>AKPDRSSFVPSLFSKKKKNVTMRSIKTTRDRVPTYQYNMNFEKLGKCIIINNKNFDKVTGMG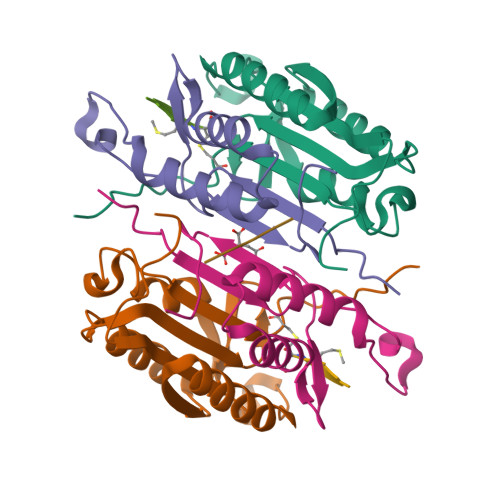VRNGTDKDAEALFKCFRSLGFDVIVYNDCSCAKMQDLLKKASEEDHTNAACFACILLSHGEENVIYGKDGVTPIKDLTAHFRGDRCKTLLEKPKLFFIQACRGTELDDGIQ[2x];>[2x]ANPRYKIPVEADFLFAYSTVPGYYSWRSPGRGSWFVQALCSILEEHGKDLEIMQILTRVNDRVARHFESQSDDPHFHEKKQIPCVVSMLTKELYFSQ;> QGHGE> MITTPLVHVASVEKGRSYEDFQKVYNAIALKLREDDEYDNYIGYGPVLVKLAWHISGTWDKHDNTGGSYGGTYRFKKEFNDPSNAGLQNGFKFLEPIHKEFPWISSGDLFSLGGVTAVQEMQGPKIPWRCGR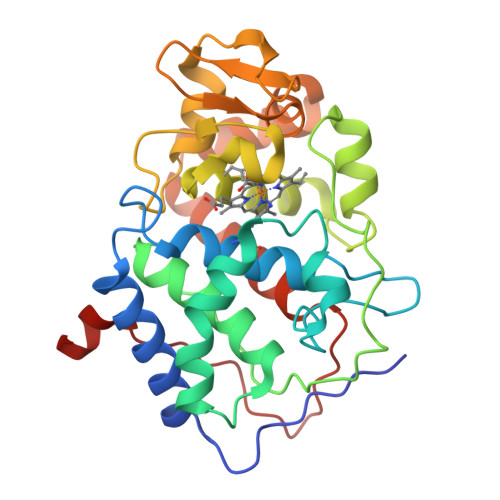VDTPEDTTPDNGRLPDADKDAGYVRTFFQRLNMNDREVVALMGAHALGKTHLKNSGYEGPWGAANNVFTNEFYLNLLNEDWKLEKNDANNEQWDSKSGYMMLPTDYSLIQDPKYLSIVKEYANDQDKFFKDFSKAFEKLLENGITFPKDAPSPFIFKTLEEQGL> MIQVTSEQWLYWLHLYFWPLLRVLALISTAPILSERAIPKRVKLGLGIMITLVIAPSLPANDTPLFSIAALWLAMQQILIGIALGFTMQFAFAAVRTAGEFIGLQMGLSFATFVDPGSHLNMPVLARIMDMLAMLLFLTFNGHLWLISLLVDTFHTLPIGSNPVNSNAFMALARAGGLIFLNGLMLALPVITLLLTLNLALGLLNRMAPQLSIFVIGFPLTLTVGIMLMAALMPLIAPFCEHLFSEIFNLLADIV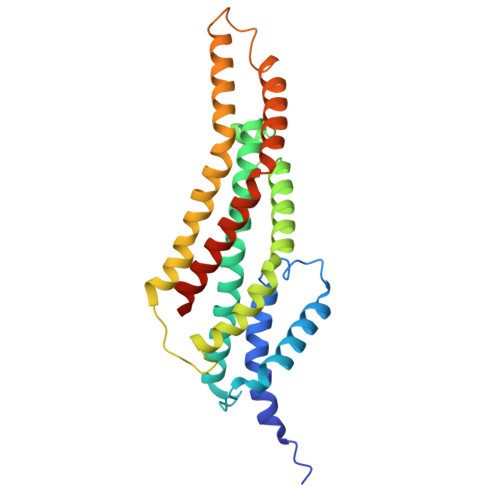SEMPINNNP> GSAKDVKFGADARALMLQGVDLLADAVAVTMGPKGRTVIIEQSWGSPKVTKDGVTVAKSIDLKDKYKNIGAKLVQDVANNTNEEAGDGTTTATVLARSIAKEGFEKISKGANPVEIRRGVMLAVDAVIAELKKQSKPVTTPEEIAQVATISANGDKEIGNIISDAMKKVGRKGVITVKDGKTLNDELEIIEGMKFDRGYISPYFINTSKGQKCEFQDAYVLLSEKKISSIQSIVPALEIANAHRKPLVIIAEDVDGEAL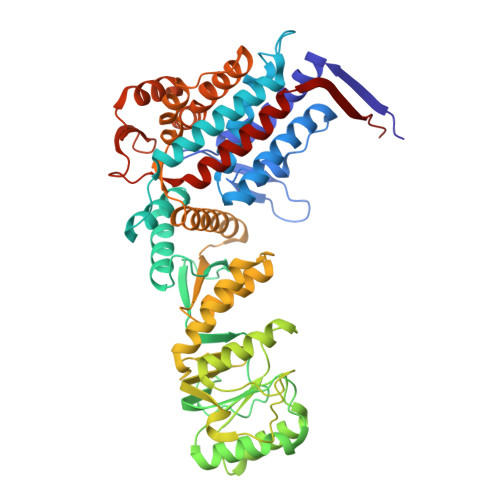STLVLNRLKVGLQVVAVKAPGFGDNRKNQLKDMAIATGGAVFGEEGLTLNLEDVQPHDLGKVGEVIVTKDDAMLLKGKGDKAQIEKRIQEIIEQLDVTTSEYEKEKLNERLAKLSDGVAVLKVGGTSDVEVNEKKDRVTDALNATRAAVEEGIVLGGGCALLRCIPALDSLTPANEDQKIGIEIIKRTLKIPAMTIAKNAGVEGSLIVEKIMQSSSEVGYDAMAGDFVNMVEKGIIDPTKVVRTALLDAAGVASLLTTAEVVVTEIPKE> GPLGSMSQSNRELVVDFLSYKLSQKGYSWSQMAAVKQALREA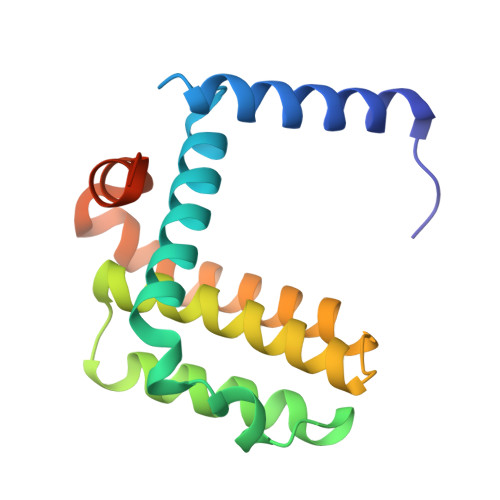GDEFELRYRRAFSDLTSQLHITPGTAYQSFEQVVNELFRDGVNWGRIVAFFSFGGALCVESVDKEMQVLVSRIAAWMATYLNDHLEPWIQENGGWDTFVELYGNNAAAESRKGQER>GPKPKNTKENLS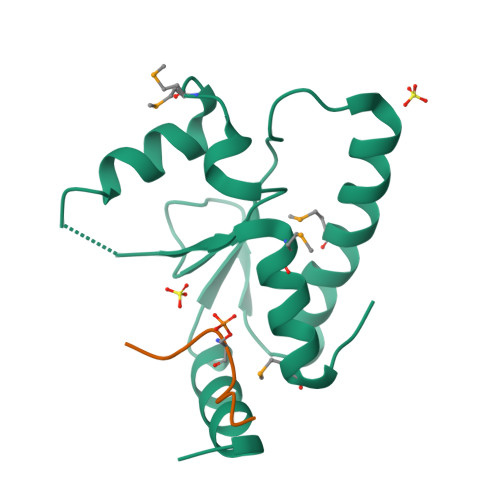KSSWRQEWLANLKLISVSLVDEFPSELSDSDRQIINEKMQLLKDIFANNLKSAISNNFRESDIIILKGEIEDYPMSSEIKIYYNELQNKPDAKKARFWSFMKTQRFVSNMGFDIQ[3x];>[3x]ESPPSLDSSPPNTSFNA> MEIPVIEPLFTKVTEDIPGAMGPVFDKNGDFYIVAPSVEVNGKPAGEILRIDLKTGKKTVICKPEVNGYGGIPAGCQCDRDANQLFVADMRLGLLVVQTDGTFEEIAKKDSEGRRMQGCAYCAFDYEGNLWITAPAGEVAPADFTISLQEKFGSIYCFTTDGQMIQVDTAFQXPAGIAVRHMNDGRPYQLIVAEQPTKKLWSYDIKGPAKIENKKVWGHIPGTHEGGAAGMDFDEDNNLLVANRGSSHIEVFGPKGGQPKMRIRCPFEKPSALHFKPQTKTIFVTEHENNAVWKFEWQRNGKKQYCETLKFGIFGSLEWSHPQFEK

Recently our laboratory has introduced a powerful mode of photochemistry into proteins, namely triplet energy transfer (EnT) photocatalysis, by developing an enantioselective [2 + 2] cyclase that relies on a genetically programmed benzophenone as a triplet sensitizer. Compared with benzophenones, thioxanthones have strong absorbance features that extend into the visible spectrum and are less susceptible to off-pathway processes that compromise EnT efficiency. Here, we develop engineered translation components to embed thioxanthone triplet sensitizers into proteins. This system enables the development of highly efficient and oxygen-tolerant photoenzymes that are powered by visible light and can achieve selective conversions that are beyond the reach of existing photocatalysts.

Following evaluation of ∼5,300 clones, a triple mutant (VEnT1.0 A21M Y37S W244R) emerged that achieves a substantial 10-fold improvement in reaction yield (2.6% to 24.8%) under the assay conditions used for evolution (70 s irradiation at 405 nm, 0.125 mol% enzyme). Pleasingly, the increased activity observed across evolution also coincided with improved selectivity, with VEnT1.3 affording (+)-1a in >99% e.e. To gain further insights into the catalytic mechanism of VEnT1.3, crystal structures of apo-VEnT1.0 and apo-VEnT1.3 were solved at 1.5-Å and 1.8-Å resolution, respectively. The structures show that the mutations installed during evolution have resulted in a repositioning of the mTX sensitizer. Interestingly in the optimized variant, mTX adopts a similar pose to the benzophenone sensitizer of EnT1.3, with the carbonyl motif projecting into the active site pocket. Molecular docking of the product (+)-1a into apo-VEnT1.3 reveals a favourable binding pose in which the product is held in a tight active site pocket shaped by mTX173, Ser37, Met21, His287, Arg244 and Gln195. In this pose, the ligand sits in close proximity to mTX (3.2 Å) in a coplanar geometry that presumably allows for efficient energy transfer between the excited sensitizer and substrate. Ligand binding is further supported by a hydrogen bond between the quinolone carbonyl and Gln195 side chain, a similar interaction to that previously observed in an EnT1.3–product complex. Mutation of Gln195 of VEnT1.3 to Ala results in a substantial reduction in activity and selectivity, providing experimental support for the predicted ligand-binding geometry and underscoring the importance of Gln195 to VEnT1.3 photocatalysis. The mTX sensitizer probably occludes one face of the quinolone substrate to direct addition of the exocyclic alkene to the 3-si face, leading to the observed stereochemical/reaction outcome.2-{5-[AMINO(IMINIO)METHYL]-1H-INDOL-2-YL}-6-(CYCLOPENTYLOXY)BENZENOLATE 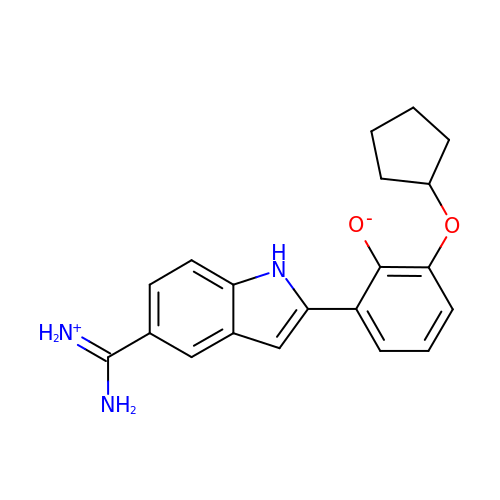| C20 H21 N3 O2 | CFSQPEBVGUSQII-UHFFFAOYSA-N>MPELPDFFEGKHFFLYGEFPGDERRRLIRYVTAFNGELEDRMNERVQFVITAQEWDPNFEEALMENPSLAFVRPRWIYSCNEKQKLLPHQLYGVVPQA[2x];>[2x]GSADETLSQTKVLLDIFTGVRLYLPPSTPDFSRLRRYFVAFDGDLVQEFDMTSATHVLGSRDKNPAAQQVSPEW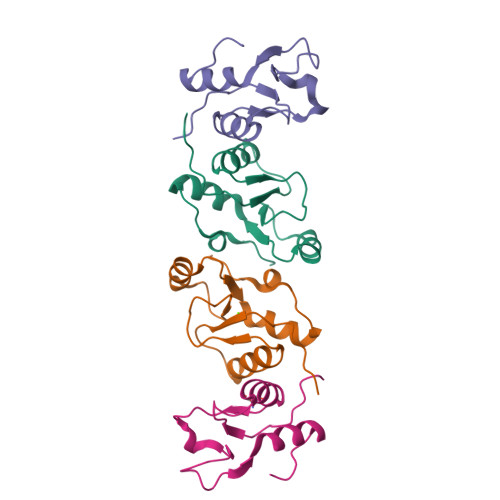IWACIRKRRLVAPS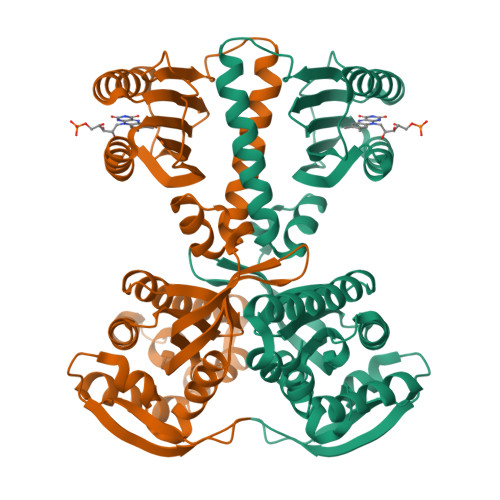> MKRLTYISKFSRPLSGDEIEAIGRISSQKNQQANVTGVLLCLDGIFFQILEGEAEKIDRIYERILADERHTDILCLKSEVEVQERMFPDWSMQTINLDENTDFLIRPIKVLLQTLTESHRILEKYTQPSIFKIISQGTNPLNIRPKAVEKIVFFSDIVSFSTFAEKLPVEEVVSVVNSYFSVCTAIITRQGGEVTKFIGDCVMAYFDGDCADQAIQASLDILMELEILRNSAPEGSPLRVLYSGIGLAKGKVIEGNIGSELKRDYTILGDAVNVAARLEALTRQLSQALVFSSEVKNSATKSWNFIWLTDSELKGKSESIDIYSIDNEMTRKSSGGLEIARNIGHYLERVGDRQPSQIFGVKSLPL4-({5-amino-1-[(2,6-difluorophenyl)carbonyl]-1H-1,2,4-triazol-3-yl}amino)benzenesulfonamide 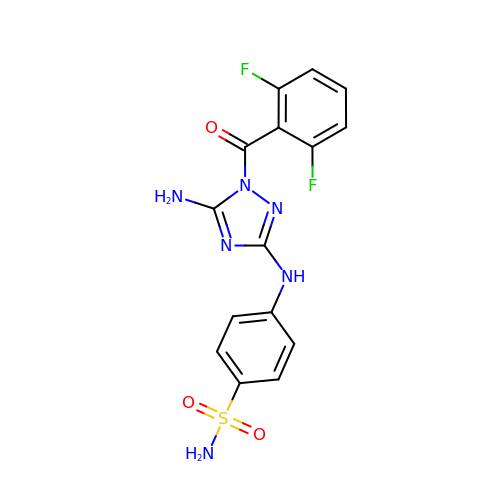| C15 H12 F2 N6 O3 S | KDKUVYLMPJIGKA-UHFFFAOYSA-N1-[4-(4-ethanoylpiperazin-1-yl)phenyl]guanidine | C13 H19 N5 O | 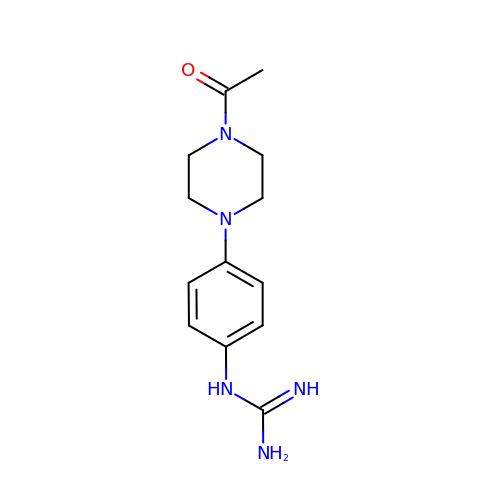MSILSEAASITEGZ-UHFFFAOYSA-N> RNRREEILQSLALMLESSDGSQRITTAKLAASVGVSEAALYRHFPSKTRMFDSLIEFIEDSLITRINLILKDEKDTTARLRLIVLLLLGFGERNPGLTRILTGHALMFEQDRLQGRINQLFE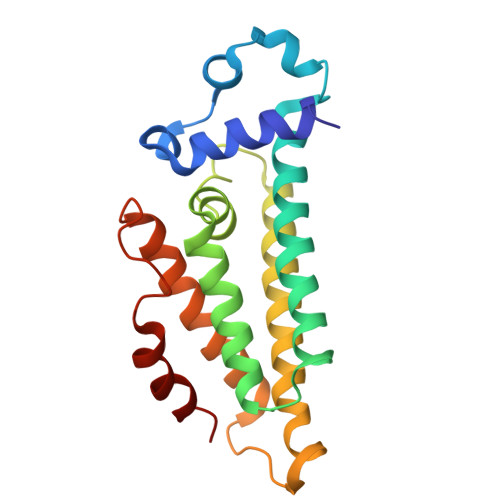RIEAQLRQVMREKRMREGEGYTTDETLLASQILAFCEGMLSRFVRSEFKYRPTDDFDARWPLIAAQLQ> MQNIKTLINRKKLLEMIPLSTRTIYNLE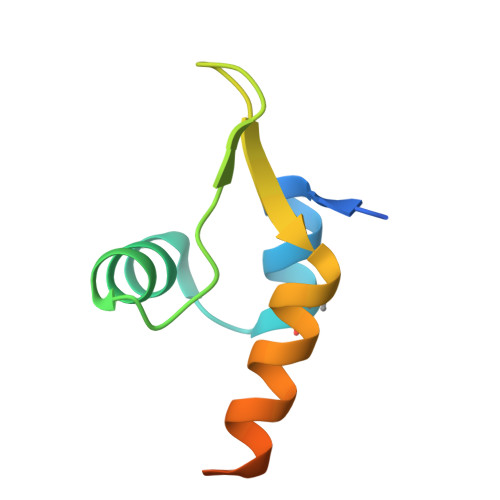QRGDFPRRIALTSRNVAWDLSEVEEWIEARKSSGDQAARPGPIEG> XSLSDKDKAAVKLLWSKISKSSDAIGNDALSRMIVVYPQTKTYFAHWPDLSPGSPHVKAHGKT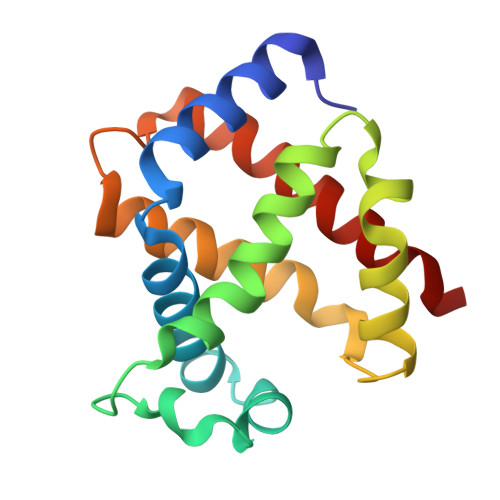VMGGIALAVSKIDDLRAGLLDLSEQHAYKLRVDPANFKILSHCILVVISMMFPKEFTPEAHVSLDKFLSGVSLALSERYR>KTFKLHEMHGLCMPNLLLNPDIHGDRIIFVCCDDLWEHDLKSGSTRKIVSNLGVINNARFFPDGRKIAIRVMRGSSLNTADLYFYNGENGEIKRITYFSGKSTGRRMFTDVAGFDPDGNLIISTDAMQPFSSMTCLYRVENDGINFVPLNLGPATHILFADGRRVIGRNTFELPHWKGYRGGTRGKIWIEVNSGAFKKIVDMSTHVSSPVIVGHRIYFITDIDGFGQIYSTDLDGKDLRKHTSFTDYYPRHLNTDGRRILFSKGGSIYIFNPDTEKIEKIEIGDLESPEDRIISIPSKFAEDFSPLDGDLIAFVSRGQAFIQDVSGTYVLKVPEPLRIRYVRRGGDTKVAFIHGTREGDFLGIYDYRTGKAEKFEENLGNVFAMGVDRNGKFAVVANDRFEIMTVDLETGKPTVIERSREAMITDFTISDNSRFIAYGFPLKHGETDGYVMQAIHVYDMEGRKIFAATTENSHDYAPAFDADSKNLYYLSYRSLDPSPDRVVLNFSFEVVSKPFVIPLIPGSPNPTKLVPRSMTSEAGEYDLNDMYKRSSPINVDPGDYRMIIPLESSILIYSVPVHGEFAAYYQGAPEKGVLLKYDVKTRKVTEVKNNLTDLRLSADRKTVMVRKDDGKIYTFPLEKPEDERTVETDKRPLVSSIHEEFLQMYDEAWKLARDNYWNEAVAKEISERIYEKYRNLVPLCKTRYDLSNVIVEMQGEYRTSHSYEMGGTFTDKDPFRSGRIACDFKLDGDHYVVAKAYAGDYSNEGEKSPIFEYGIDPTGYLIEDIDGETVGAGSNIYRVLSEKAGTSARIRLSGKGGDKRDLMIDILDDDRFIRYRSWVEANRRYVHERSKGTIGYIHIPD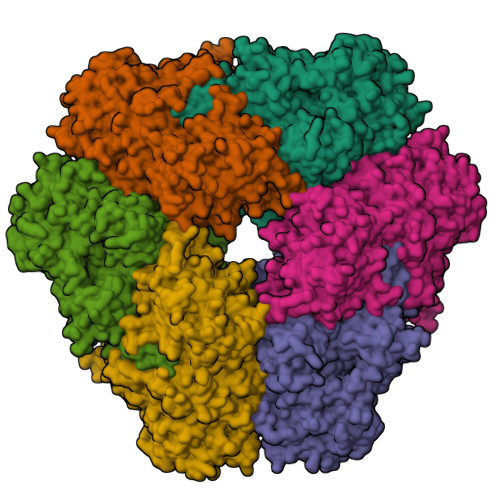MGMMGLNEFYRLFINESSYQGLIVDVRFNGGGFVSQLIIEKLMNKRIGYDNPRRGTLSPYPTNSVRGKIIAITNEYAGSDGDIFSFSFKKLGLGKLIGTRTWGGVVGITPKRRLIDGTVLTQPEFAFWFRDAGFGVENYGVDPDVEIEYAPHDYLSGKDPQIDYAIDALIEELRNWNEELPQRPS[6x]>EACRDGLR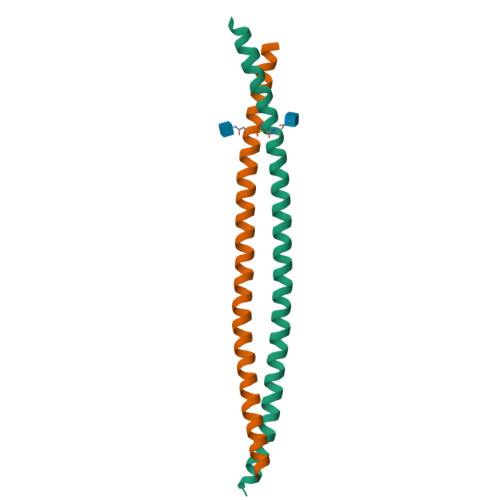AVMECRNVTHLLQQELTEAQKGFQDVEAQAATCNHTVMALMASLDAEKAQGQKKVEELEGEITTLNHKLQDASAEVERLRRENQVLSVRIADKGT[2x]>MKIRDLLKARRGPLFSFEFFPPKDPEGEEALFRTLEELKAFRPAFVSITYGAMGSTRERSVAWAQRIQSLGLNPLAHLTVAGQSRKEVAEVLHRFVESGVENLLALRGDPPRGERVFRPHPEGFRYAAELVALIRERY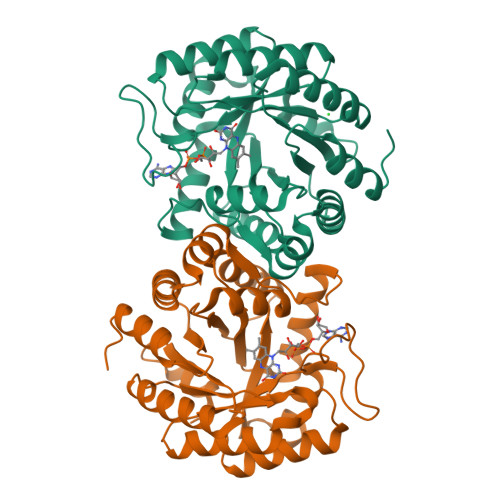GDRVSVGGAAYPEGHPESESLEADLRHFKAKVEAGLDFAITQLFFNNAHYFGFLERARRAGIGIPILPGIMPVTSYRQLRRFTEVCGASIPGPLLAKLERHQDDPKAVLEIGVEHAVRQVAELLEAGVEGVHFYTLNKSPATRMVLERLGLRPASGQPAKLAAALEHHHHHH[8x]> QVASEYLGGPGGDAFDDKAVAQNGDITRIEMQCTDVATYIKLRYGKVDSRQWGWGNE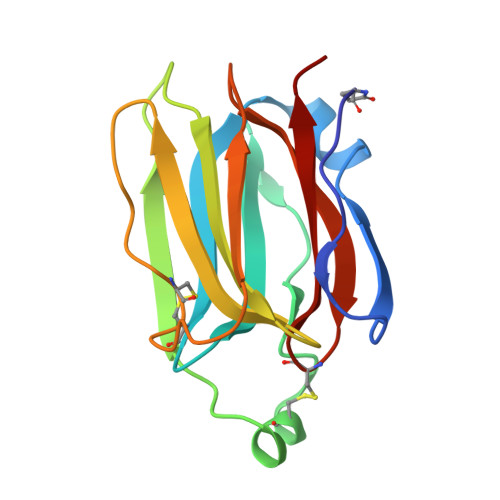NCIQWSKKGEKVVHELSSGEYITSAIVTYGKYVQSITFKTNKRTLPRCGTSATEKSVTVLIPGGLKYISGRWGCRIDGLRFHAKC> NDLVFSSWGGTTQDAQKAAWAEKFMVETGINVLQDGPTDYGKLKAMVEANGVTWDVVDVEGDYAAQAGPKGLLEKLDFSVIDKTKLDPRFVTDYSVGSFYYSFVIGCNVDSVSACPKSWADLFDTAKFPGKRTFYKWSAPGVIEAALLADGVTADKLYPLDLDRAFKKLDTIKSDIIWWSGGAQSQQLIASAEAPFGSVWNGRMTALEQSGVKVETSWAQNITAADSL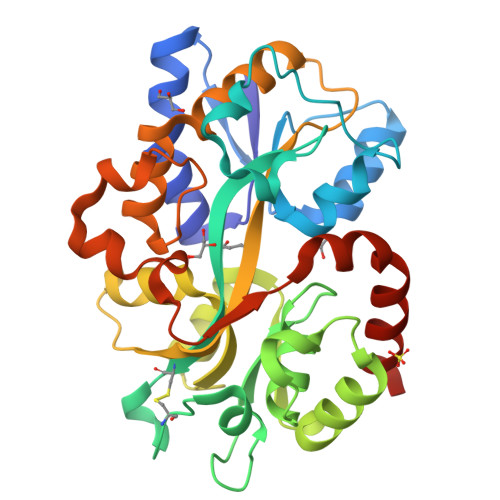VVPKGTKNKDAAMKFIALATSAQAQADMATATGYAPVNIESAKLMDPKIAKSLPDQQTESQVNADMNYWAQHRDEIGERWYAWQAKHHHHHH>GSMSFIPVAEDSDFPIQNLPYGVFSTQSNPKPRIGVAIGDQILDLSVIKHLFTGPALSKHQHVFDETTLNNFMGLGQAAWKEARASLQNLLSASQARLRDDKELRQRAFTSQASATMHLPATIGDYTDFYSSRQHATNVGIMFRGKENALLPNWLHLPVGYHGRASSIVVSGTPIRRPMGQMRPDNSKPPVYGACRLLDMELEMAFFVGPGNRFGEPIPISKAHEHIFGMVLMNDWSARDIQQWEYVPLGPFLGKSFGTTISPWVVPMDALMPFVVPNPKQDPKPLPYLCHSQPYTFDINLSVSLKGEGMSQAATICRSNFKHMYWTMLQQLTHHSVNGCNLRPGDLLASGTISGSDPESFGSMLELSWKGTKAIDVGQGQTRTFLLDGDE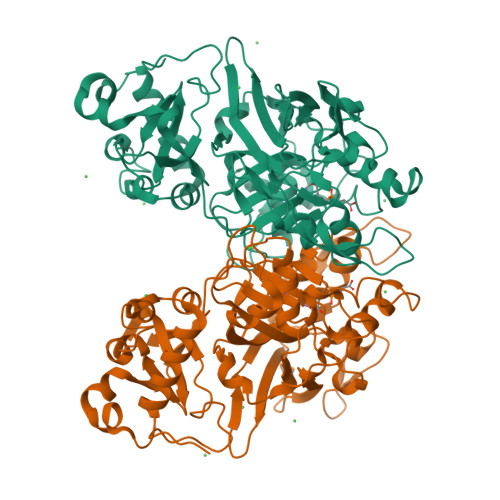VIITGHCQGDGYRVGFGQCAGKVLPALSPA[2x]>MADQAMTDQDQGAVTLYSGTAITDAKKNHPFSVKVGLAQVLRGGAIVEVSSVNQAKLAESAGACSVIVSDPVRSRGGVRRMPDPVLIKEVKRAVSVPVMARARVGHFVEAQILESLAVDYIDESEIISVADDDHFINKHNFRSPFICGCRDTGEALRRIREGAAMIRIQGDLTATGNIAETVKNVRSLMGEVRVLNNMDDDEVFTFAKKISAPYDLVAQTKQMGRVPVVQFASGGITTPADAALMMQLGCDGVFVGSEVFDGPDPFKKLRSIVQAVQHYNDPHVLAEMSSGLENAMESLNVRGDRIQDFGQGSV[4x];>MEGTGVVAVYGNGAITEAKKSPFSVKVGLAQMLRGGVIMDVVNAEQARIAEEAGACAVMALERVPADIRAQGGVARMSDPQMIKEIKQAVTIPVMAAARIGHFVEAQILEAIGIDYIDESEVLTLADEDHHINKHNFRIPFVC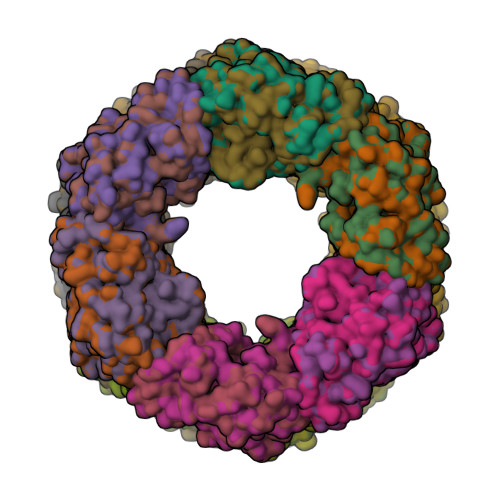GCRNLGEALRRIREGAAMIRTKGEAGTGNIIEAVRHVRSVNGDIRVLRNMDDDEVFTFAKKLAAPYDLVMQTKQLGRLPVVQFAAGGVATPADAALMMQLGCDGVFVGSGIFKSGDPARRARAIVQAVTHYSDPEMLVEVSCGLGEAMVGINLNDEKVERFANRSEHHHHHH[4x]>SIDYVEMAVNKRTVRMPHQLFIGGEFVDAEGAKTSETINPTDGSVICQVSLAQVTDVDKAVAAAKDAFENGRWGKISARDRGRLMYRLADLMEQHQEELATIEALDAGAVYTLALKTHVGMSIQTFRYFAGWCDKIQGSTIPINQARPNRNLTLTRKEPVGVCGIIIPWNYPLMMLSWKTAACLAAGNTVVIKPAQVTPLTALKFAELTLKAGIPKGVVNVLPGSGSLVGQRLSDHPDVRKIGFTGSTEVGKHIMKSCAISNVKKVSLELGGKSPLIIFADCDLNKAVQMGMSSVFFNKGENCIAAGRLFVEDSIHDEFVRRVVEEVRKMKVGNPLDRDTDHGPQNHHAHLVKLMEYCQHGVKEGATLVCGGNQVPRPGFFFEPTVFTDVEDHMFIAKEESFGPVMIISRFADGDLDAVLSRANATEFGLASGVFTRDINKALYVSDKLQAGTVFVNTYNKTDVAAPFGGFKQSGFGKDLGEAALNE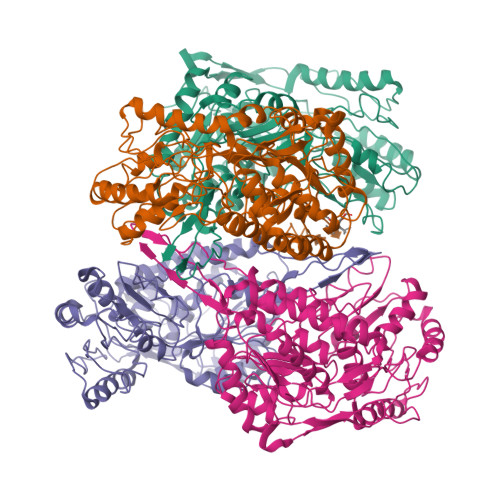YLRVKTVTFEY[4x]> XUGCUGGCUAAGGXCCGAAAGG;> CUAUGCCUGCUG

The TNA backbone is composed of phosphodiester-linked 3′→2′ α-l-threofuranose sugars and, therefore, has one fewer atom in its repeating unit than RNA. Critically, TNA can form stable Watson−Crick duplexes with itself, DNA and RNA, such that the exchange of genetic information between these polymers appears feasible. Here, we examine the behaviour of TNA in nonenzymatic template-directed primer extension reactions from both a kinetic and a structural perspective. Taken together, we propose that structural constraints explain the diminished ability of TNA to engage in nonenzymatic template-directed primer extension, and we discuss the consequences of these observations for the plausibility of the involvement of TNA in the origin of primitive cells.

To gain structural insight into the conformation of the reaction center in TNA-templated nonenzymatic primer extension, we co-crystallized and determined the structure of an RNA hairpin complex, similar to that used above, but this time containing a single TNA residue on the template strand of a gapped stem. The RNA hairpin-monomer complex (TNA-T1) contains a single tG residue at the appropriate position to serve as the template to bind a free CMP monomer. The TNA-T1 complex also crystallized in the R3 space group, and we determined the structure to a resolution of 2.95 Å. The tG residue on the template strand is well-ordered, forming three hydrogen bonds with the bound CMP monomer through a Watson-Crick base-pairing interaction. The tG threose sugar ring is in the C4′-exo conformation, and the glycosidic torsion angle χ of tG is –111°, similar to the tA residue seen at the end of the primer. However, the noncovalently bound CMP is poorly ordered, suggesting a significant degree of conformational heterogeneity. The electron density of the monomer's sugar and phosphate is poorly resolved, yielding only a rough estimate of 4 Å for the distance between the 3′-OH of primer and the P atom of the CMP. The tG threose sugar, constrained by stacked upstream and downstream RNA nucleotides, is shifted by 1.1–1.7 Å compared to the native RNA ribose sugar ring. As expected, the tG residues in the TNA-P1 and TNA-T1 complexes share similar α and γ torsion angles, likely due to similar structural constraints on the threo-nucleotide residue in the RNA context of both hairpin structures. Overall, a single TNA nucleotide substitution on the template does not dramatically disrupt the RNA structure.> AWSVNNFLMTGPKAYLTYSASVAVGAQNGIEECKYQFAWERWNCPESTLQLATHNGLRSATRETSFVHAISSAGVMYTLTRNCSMGDFDNCGCDDSRNGRIGGRGWVWGGCSDNAEFGERISKLFVDGLETGQDARALMNLHNNEAGRLAVKETMKRTCKCHGISGSCSIQTCWLQLAEFRDIGNHLKIKHDQALKLEMDKRKMRSGNSADNRGAIADAFSSVAGSELIFLEDSPDYCLKNISLGLQGTEGRECLQSGKNLSQWERR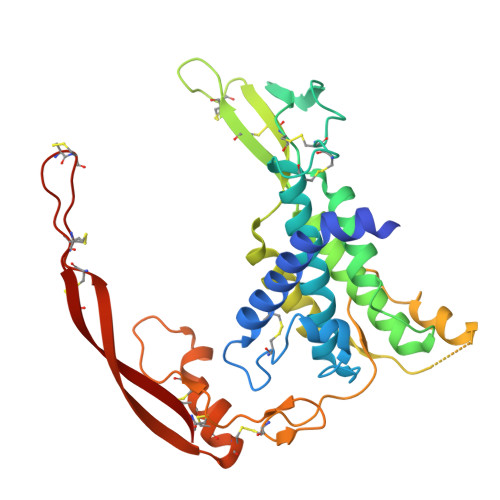SCKRLCTDCGLRVEEKKTEIISSCNCKFHWCCTVKCEQCKQVVIKHFCA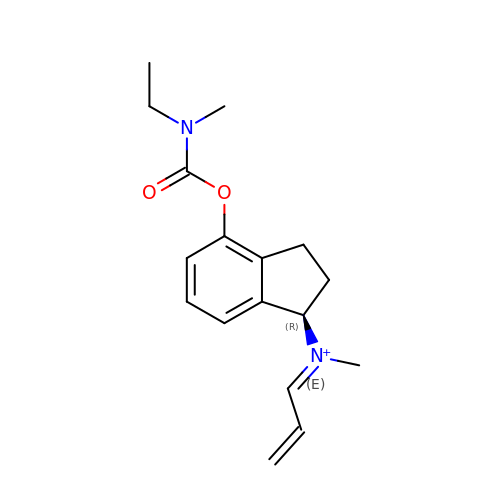(1R)-4-({[ETHYL(METHYL)AMINO]CARBONYL}OXY)-N-METHYL-N-[(1E)-PROP-2-EN-1-YLIDENE]INDAN-1-AMINIUM | C17 H23 N2 O2 | OETCNLZUDQXQBD-IYSPOMMRSA-N> MEEVEQTPLQEALNQLMRQLQRKDPSAFFSFPVTDFIAPGYSMIIKHPMDFSTMKEKIKNNDYQSIEELKDNFKLMCTNAM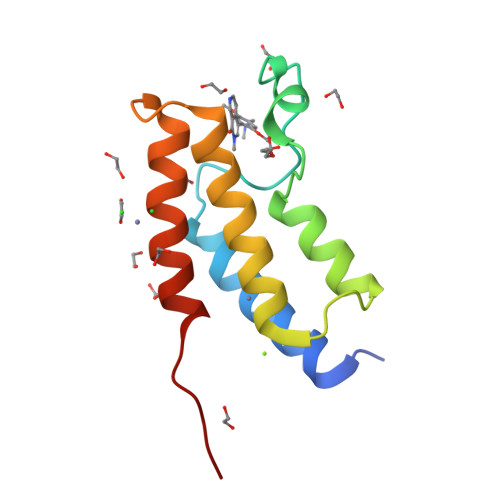IYNKPETIYYKAAKKLLHSGMKILSQERIQS>[3x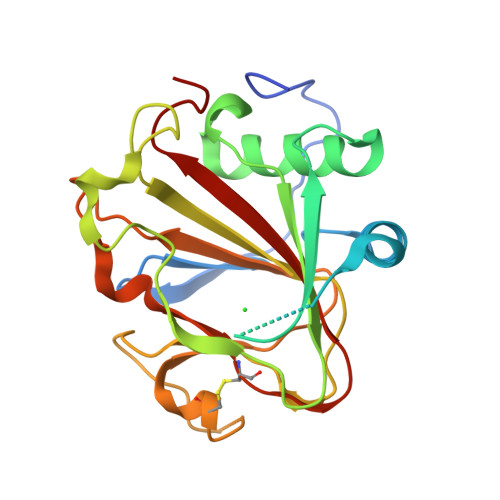]MHHHHHHMVGFGELKEEWRGEVVHLSWSPRAFLLKNFLSDEECDYIVEKARPKMVKSSVVDNESGKSVDSEIRTSTGTWFAKGEDSVISKIEKRVAQVTMIPLENHEGLQVLHYHDGQKYEPHYDYFHDPVNAGPEHGGQRVVTMLMYLTTVEEGGETVLPNAEQKVTGDGWSECAKRGLAVKPIKGDALMFYSLKPDGSNDPASLHGSCPTLKGDKWSATKWIHVAPIGGRH6-{8-[(1,3-benzothiazol-2-yl)carbamoyl]-3,4-dihydroisoquinolin-2(1H)-yl}-3-{1-[(pyridin-4-yl)methyl]-1H-pyrazol-4-yl}pyridine-2-carboxylic 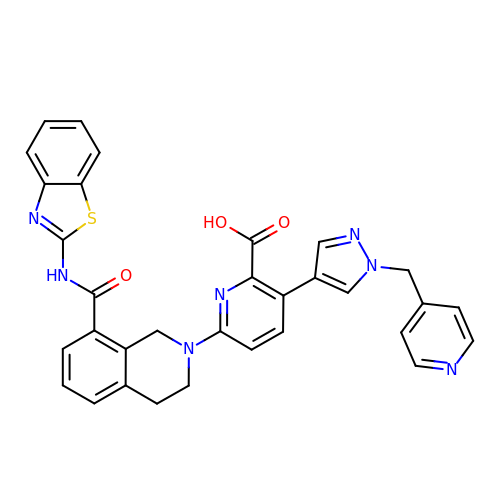acid | C32 H25 N7 O3 S | WBCFKELVKOCTOB-UHFFFAOYSA-N> PSGFNVVIEHDSEYQPDVKVTYYKNSIGTEANGFDTGPVFGGERIYNLASSLSYIRNKINVELPSVYAMAGEVVNNGNELLLINGTEIMRFVIEGATITKGYVEKVKPPTNLIVSDVTSTSAKISWENGG;> MADKNYLHTAYANSADGTDGFTTVYPNLNLLVNSSAKNKEGFFKNFDKVENGYGEVTMKGTNAWVNKDLGEGFSIQPINYKPGDKYTMSVDVMFTSWNVPAGTTISAFWMRQRYTENSWKEICTIDLPKDPSKMLNQWIRITQTSTIPPYEDPSVGTQAILNVGFFGQQEGSFTIRVRNPKQELGSIATPYMPSASEVTTADWPKFVGTYVDTNPVSSTVSSKYDWDEMKYRVYLDGTPVGGSKLLSFDLENLKAGTSYNVQVSQINGNVESDKSESVAFKTTLPK;> AELTKITRGMQNGAETINDNLNKLNTITVQKTGDETIAGKKTFSGDVSVDGDFTMKKFADSYVAFFANKGSGNTVTFTAPWDCTAEVELFYHGWGYSGGEWEIGITTPSGLTQIYEATGYTNGHDNQAISMPTKAIYSGLKKGLQYTFDIRDANGRGGGPKHPMMIVKLYRNA;>MAELTKITRGMQNGAETINDNLNKLNTITVQKTGDETIAGKKTFSGDVSVDGDFTMKKFADSYVAFFANKGSGNTVTFTAPWDCTAEVELFYHGWGYSGGEWEIGITT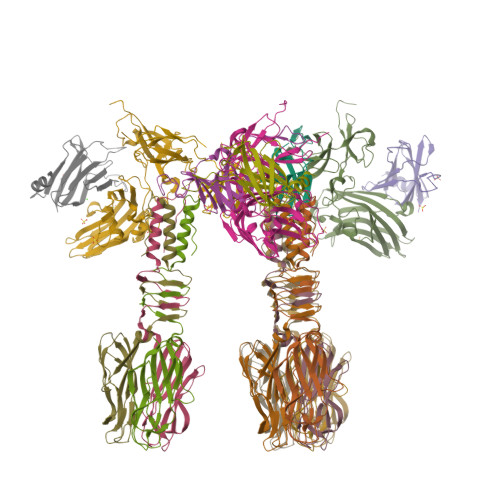PSGLTQIYEATGYTNGHDNQAISMPTKAIYSGLKKGLQYTFDIRDANGRGGGPKHPMMIVKLYRNA[3x]> SGISLDNSYKMDYPEMGLCIIINNKNFHKSTGMTSRSGTDVDAANLRETFRNLKYEVRNKNDLTREEIVELMRDVSKEDHSKRSSFVCVLLSHGEEGIIFGTNGPVDLKKITNFFRGDRCRSLTGKPKLFIIQACRGTELDCGIETD;> ASGVADDMACHKIPVEADFLYAYSTAPGYYSWRNSKDGSWFIQSLCAMLKQYA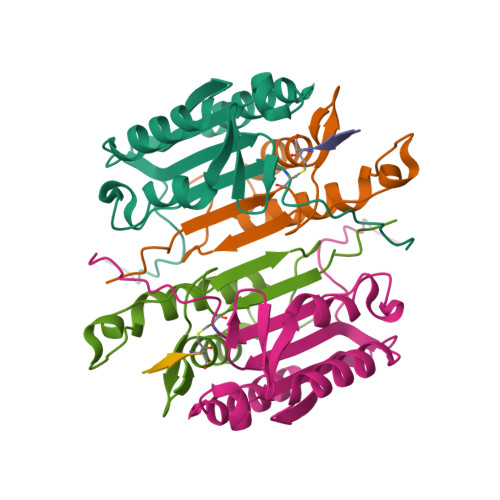DKLEFMHILTRVNRKVATEFESFSFDATFHAKKQIPCIVSMLTKELYFYH> SGSMTWRRFDVAYHDPDLDRLILAARPLLSESPGRSWFQRHWVRGPHLELWFDHPEPSWERVREVLGTHLRAHPSRTRIDPDRLLPQHRRLALAEQIDEPLLPFYDDNTLHRAVPRSRVHVLGSAAAEDLFHDFHAAASTAAFDQLDAVVAGESRLGLAFELMIAAAHAHAEGGITGGFVSFRSHAEAFLAGAAGLRERWEAEYRTRAEALRAQVAAVVTGTPRGRAWTGLLDGFAGRGDELIASGALTVEPASPTAAAEPDTEFHRALRANRTWHDEVLRSPSFRRYRLLL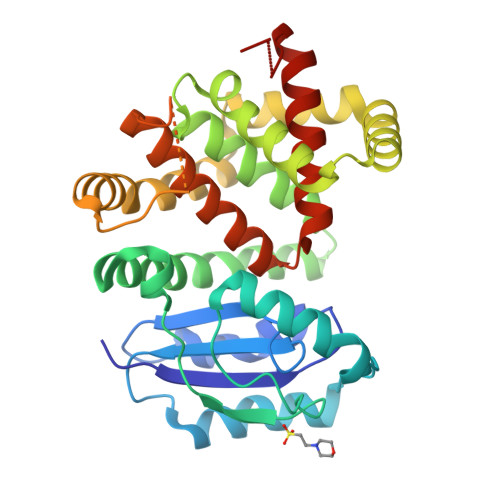NLTYLQMSRLGVTAVQRSLLCHFAASAVEEEYGVSAIEIAVGGM>[3x]MIERLVTLCFNRRGIVALVFAMVALYGWYAWKQLPLEAYPDIADTTSQVVTQVNGLAAEEVEQQITIPLEREIMGVPGMHVMRSKSTFGLSLITVVFKDGAEDYWSRQRLQERINGVSLPYGAQPSLDPLTSPIGEIYRYTLVSKTRDLRELSELQFWKVIPRLKQVAGVVDVANFGGLTTQFMLEFDPVMLSKYNISLNQITQAISENNANAGGSILNRGEQGLVVRGVGLIRNLDDLGNIVVTQKNGVPVLVKDLGRVVLGNPQRHGIL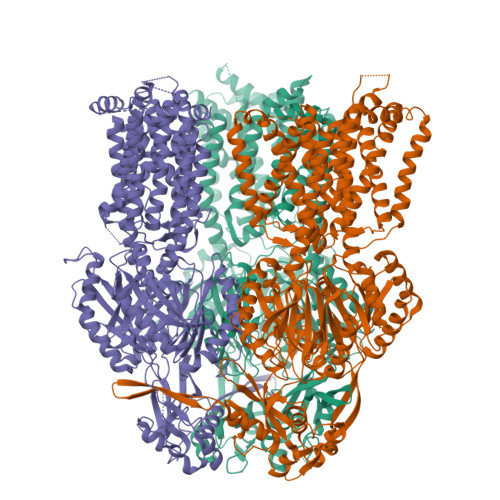GMDRNPDTIQGITLLLKNENPSVVMEGVHAAVRDLNDNILPKDVKVVPYIDRSNLVDATVHTVGKTLMEGMFLVSLVLLLFLGSPRAAIIVAVTIPLSLLMAFILMHHFKIPANLLSLGAIDFGIIVDGAIVVMENILRRREEDAEKELHGRDIMQSVLQVARPIFFGMIVIITAYLPLFAFQRIEYKLFSPMAFAVGFALFGALLVALLLIPGLAYWAYRKPRKVFHNPALVWLAPRYESVLNRLVGSTRTAIGIAVATLVGVMILGATIGRDFLPYLDEGSIWLQVTLPPGISLEKAGQMADNLRAATMEFPEVEHVVTQVGRNDEGTDPFSPSHIETAVTLHPYSTWTSGRDKQQLIEAMATRFRDLPGTQVGFSQPMIDGVLDKLAGAHSDLVVKVYGNDFAETRQVATAITRLLKTVPGAQDVIIDQEPPLPQVRIDVDRAAAARLGINVADVMALIQTGIGGSPVTQVFVEDRSYNVVARFIGSSRNDPEAIGNLTLTAANGAHVALAQVAHIRLAEGETTITREMNKRHLTVRLNLRGRDLSTFLEEARMRIDKEVPYDRTHIQVAWGGQFENQQRAQARLAVILPMVLALMFVLLFGEFKNLRQPALILMAVPLATLGGLVALHLRGMTLNVSSAVGFIALFGVAVLNAIIMIANLNRWRDTSGVSLKEAVVRGAGERMRPVLMTATVAALGLIPAALAHGLGSDVQRPLATVVVGGLITATALTLVLLPALYYLIETRAAKQVREEPPVQFGPTSEGDLHHHHHH> EEAPWPPPEGAFVGFVLSRKEPMWADLLALAAARGGRVHRAPEPYKALRDLKEARGLLAKDLSVLALREGLGLPPGDDPMLLAYLLDPSNTTPEGVARRYGGEWTEEAGERAALSERLFANLWGRLEGEERLLWLYREVERPLSAVLAHMEATGVRLDVAYLRALSLEVAEEIARLEAEVFRLAGHPFNLNSRDQLERVLFDELGLPAIGKTEKTGKRSTSAAVLEALREAHPIVEKILQYRELTKLKSTYIDPLPDLIHPRTGRLHTRFNQTATATGRLSSSDPNLQNIPVRTPLGQRIRRAFIAEEGWLLVALDYSQIELRVLAHLSGDENLIRVFQEGRDIHTETASWMFGVPREAVDPLMRRAAKTINFGVLYGMSAHRLSQELAIPYEEAQAFIERYFQSFPKVRAWIEKTLEEGRRRGYVETLFGR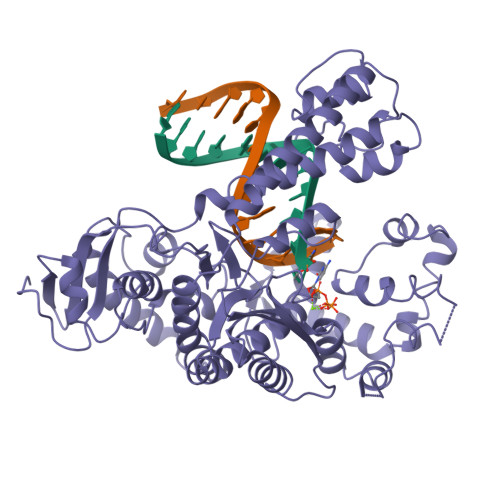RRYVPDLEARVKSVREAAERMAFNMPVQGTAADLMKLAMVKLFPRLEEMGARMLLQVHDELVLEAPKERAEAVARLAKEVMEGVYPLAVPLEVEVGIGEDWLSAKE(5R)-5-[(1E)-BUTA-1,3-DIENYL]-4-HYDROXY-3,5-DIMETHYLTHIOPHEN-2(5H)-ONE | C10 H12 O2 S | 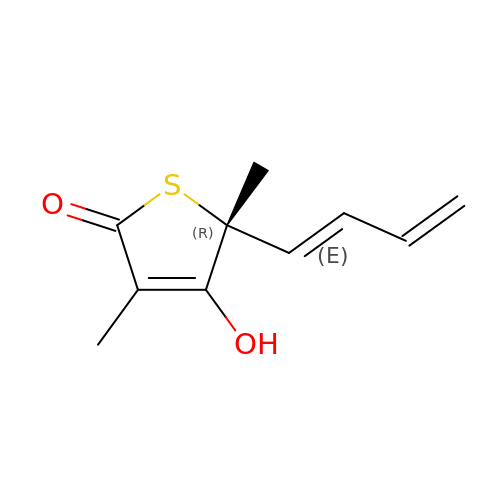TXGVAQMIEXZDPM-BRAIEQGRSA-N>MSQHNEKNPHQHQSPLHDSSEAKPGMDSLAPEDGSHRPAAEPTPPGAQPTAPGSLKAPDTRNEKLNSLEDVRKGSENYALTTNQGVRIADDQNSLRAGSRGPTLLEDFILREKITHFDHERIPERIVHARGSAAHGYFQPYKSLSDITKADFLSDPNKITPVFVRFSTVQGGAGSADTVRDIRGFATKFYTEEGIFDLVGNNTPIFFIQDAHKFPDFVHAVKPEPHWAIPQGQSAHDTFWDYVSLQPETLHNVMWAMSDRGIPRSYRTMEGFGIHTFRLINAEGKATFVRFHWKPLAGKASLVWDEAQKLTGRDPDFHRRELWEAIEAGDFPEYELGFQLIPEEDEFKFDFDLLDPTKLIPEELVPVQRVGK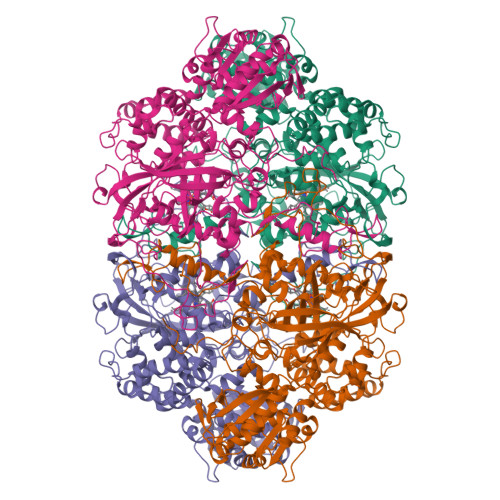MVLNRNPDNFFAENEQAAFHPGHIVPGLDFTNDPLLQGRLFSYTDTQISRLGGPNFHEIPINRPTCPYHNFQRDGMHRMGIDTNPANYEPNSINDNWPRETPPGPKRGGFESYQERVEGNKVRERSPSFGEYYSHPRLFWLSQTPFEQRHIVDGFSFQLSKVVRPYIRERVVDQLAHIDLTLAQAVAKNLGIELTDDQLNITPPPDVNGLKKDPSLSLYAIPDGDVKGRVVAILLNDEVRSADLLAILKALKAKGVHAKLLYSRMGEVTADDGTVLPIAATFAGAPSLTVDAVIVPCGNIADIADNGDANYYLMEAYKHLKPIALAGDARKFKATIKIADQGEEGIVEADSADGSFMDELLTLMAAHRVWSRIPKIDKIPA[4x]2-methoxy-6-propyl-N-(2-{4-[(1H-tetrazol-5-yl)methoxy]phenyl}ethyl)thieno[2,3-d]pyrimidin-4-amine | C20 H23 N7 O2 S | 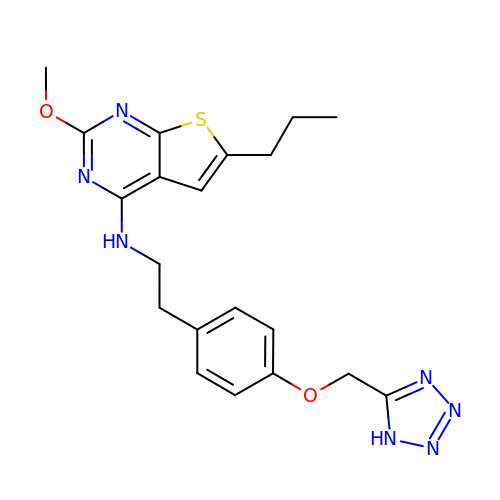ACCUSJFCOLLWHH-UHFFFAOYSA-N> MASEAIKGAVVGIDLGTTNSCVAVMEGKQAKVLENAEGARTTPSVVAFTADGERLVGMPAKRQAVTNPNNTFYATKRLIGWRYDDPEVQKDIKNVPFKIVRASNGDAWVEAHGKLYSPSQIGAFVLMKMKETAENYLGHTAKNAVITVPAYFNDSQRQATKDAGQISGLNVLRVINEP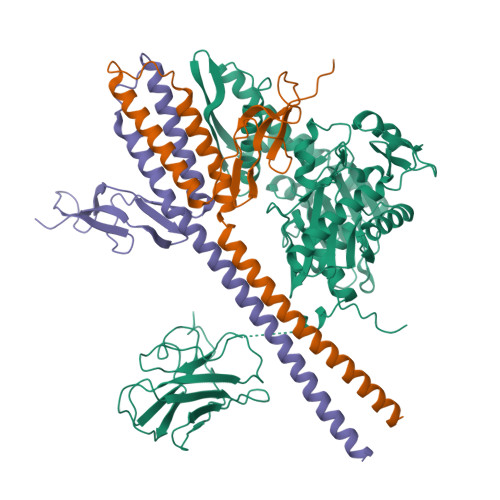TAAALAYGLDKSEDKVIAVYDLGGGTFDISILEIQKGVFEVKSTNGDTFLGGEDFDQALLRHIVKEFKRETGVDLTKDNMALQRVREAAEKAKCELSSSVQTDINLPYLTMDSSGPKHLNMKLTRAQFEGIVTDLIRRTIAPCQKAMQDAEVSKSDIGEVILVGGMTRMPKVQQTVQDLFGRAPSKAVNPDEAVAIGAAIQGGVLAGDVTDVLLLDVTPLSLGIETLGGVFTKLINRNTTIPTKKSQVFSTAADGQTQVEIKVCQGEREMAGDNKLLGQFTLIGIPPAPRGVPQIEVTFDIDANGIVHVSAKDKGTGREQQIVIQSSGGLSKDDIE;>[2x]TLLEEKVKLEEQLKETVEKYKRALADTENLRQRSQKLVEEAKLYGIQAFCKDLLEVADVLEKATQCVPKEEIKDDNPHLKNLYEGLVMTEVQIQKVFTKHGLLKLNPVGAKFDPAEHEALFHTPVEGKEPGTVALVSKVGYKLHGRTLRPALVGVVKEASA The Pat1 protein is involved in different aspects of mRNA decapping activation. Hence, Pat1 is considered as a central platform protein for decapping. Indeed, the crystal structure of the S. cerevisiae Pat1C shows that this domain structurally belongs to the ARM repeat superfamily, which mostly encompasses proteins involved in protein-protein interaction. In conclusion, the crystal structure of the ScPat1 C-terminal domain has revealed two functionally important regions localized at opposite extremities of the domain.

We therefore cloned the ScPat1C (473-796) domain, over-expressed it in E. coli and purified it in milligram amounts to homogeneity. The SeMet labeled and unlabeled proteins crystallized in three different space groups. Only structures refined to higher resolution (crystal forms II and III) will be discussed in this manuscript. Three and two copies of the ScPat1C molecule are present in the asymmetric unit of crystal forms II and III, respectively. All these structures can be superimposed onto each other with rmsd values ranging from 0.3 Å to 1.2 Å over 260-310 Cα atoms. The relatively high rmsd values observed between some molecules result from flexibility of both N- and C-terminal extremities of this domain. This flexibility is also supported by the observation that residues 484-524 from one protomer as well as residues 788-796 (corresponding to a β-sheet, see below) from another one are ill-defined in the electron density maps and hence absent from the final model. The crystal packing radically differs between crystal forms II and III. ScPat1C is organized as an array of 5 repeats of 3 helices stacked against each other to form a solenoid structure. The fifth and final motif is capped at its C-terminal end by helix α15 followed by a two-stranded anti-parallel β-hairpin, which folds back onto helices α14 and α15.

>GGKKFILELIETVYEEILDLEANLRNGQQTDSTAMWEALHIDDSSYDVNPFISMLSFDKGIKIMPRIFNFLDKQQKLKILQKIFNELSHLQIIILSSYKTTPKPTLTQLKKVDLFQMIILKIIVSFLSNNSNFIEIMGLLLQLIRNNNVSFLTTSKIGLNLITILISRAALIKQDSSRSNILSSPEISTWNEIYDKLFTSLESKIQLIFPPREYNDHIMRLQNDKFMDEAYIWQFLASLALSGKLNHQRIIIDEVRDEIFATINEAETLQKKEKELSVLPQRSQELDTELKSIIYNKEKLYQDLNLFLNVMGLVYRDGEISELKHHHHHH[3x]> RCCHPQCGAVEE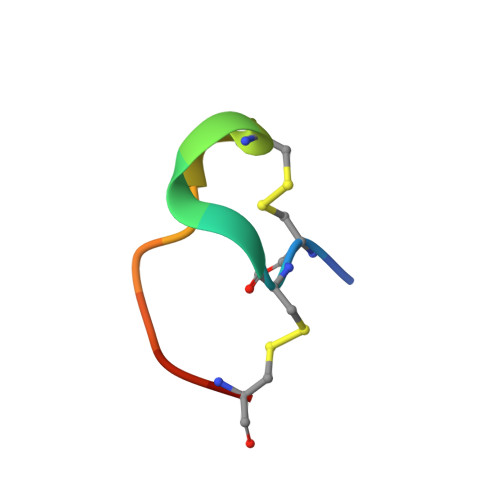CR> ATAAEIAALPRQKVELVDPPFVHAHSQVAEGGPKVVEFTMVIEEKKIVIDDAGTEVHAMAFNGTVPGPLMVVHQDDYLELTLINPETNTLMHNIDFHAATGALGGGGLTEINPGEKTILRFKATKPGVFVYHCAPPGMVPWHVVSGMNGAIMVLPREGLHDGKGKALTYDKIYYVGEQDFYVPRDENGKYKKYEAPGDA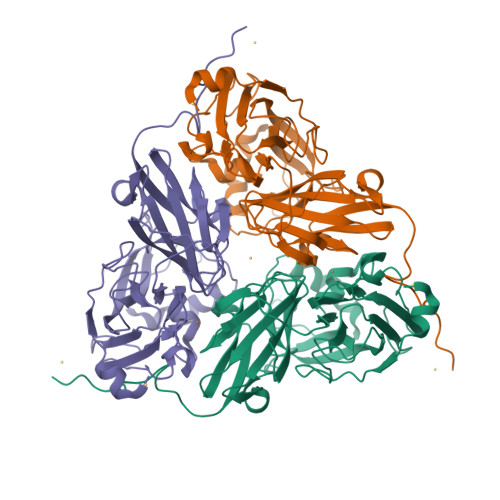YEDTVKVMRTLTPTHVVFNGAVGALTGDKAMTAAVGEKVLIVHSQANRDTRPDLIGGHGDYVWATGKFNTPPDVDQETWFIPGGAAGAAFYTFQQPGIYAYVNHNLIEAFELGAAAHFKVTGEWNDDLMTSVLAPSGTIEGR> MAHHHHHHSSGLEVLFQGPQIPLCANLVPVPITNATLDRITGKWFYIASAFRNEEYNKSVQEIQATFFYFTPNKTEDTIFLREYQTRQNQCFY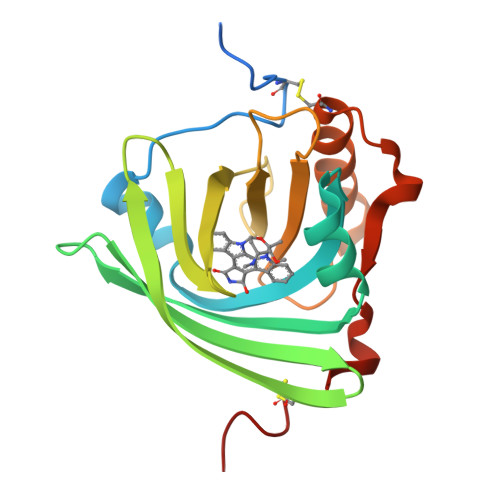NSSYLNVQRENGTVSRYEGGREHVAHLLFLRDTKTLMFGSYLDDEKNWGLSFYADKPETTKEQLGEFYEALDCLRIPRSDVMYTDWKKDKCEPLEKQH>[2x]MGSSHHHHHHSQDPMSQLTYDDSFLLDGKEIRLLSGAMHYFRTVPEYWEDRLLKLKACGFNTVETYVAWNLHEPEEGQFVFEGIADIVRFIKTAEKVGLHVIVRPGPFICAEWEFGGFPYWLLTVPNIKLRCFNQPYLEKVDAYFDVLFERLRPLLSSNGGPIIALQIENEYGSFGNDQKYLQYLRDGIKKRVGNELLFTSDGPEPSMLSGGMIEGIFETVNFGSRAESAFAQLKQYQPNAPLMCMEFWHGWFDHWGEEHHTRSAESVVETLEEILKQNGSVNFYMAHGGTNFGFYNGANHNETDYQPTITSYDYDGLLTESGDVTEKFYAVRKVFEKYVDLPELNLPAPIPKRLFGKVKFTEHAGLLDSLHRISTPQKSEAPLPMEKYGQAYGFIVYETTIKGAYGKQALTVQDIHDRGQVYVNGEYVGIVERNRGCSRLVVE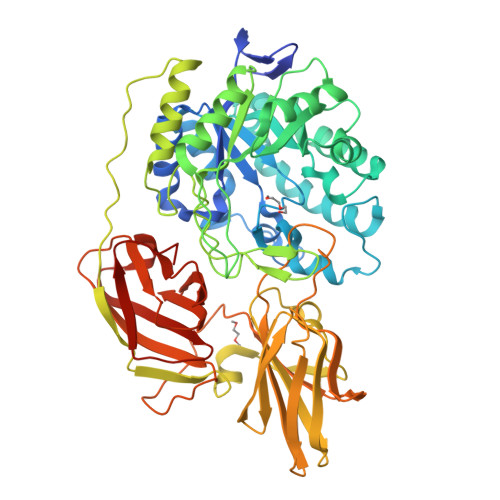LTEEESKLQIIVENMGRINYGPFVVDYKGITEGVRLGNQFLFDWTVYPLPLKDLSSLEFTADEVKENFPYFHKGILTVDKAADTFIDLSEWTKGVVFVNGHHLGRYWEIGPQQTLYVPAPFLQEGENEIILLELHKHHQSVTFVDTPVLGAIPKTP> GSMGKPFFTRNPSELKGKFIHTKLRKSSRGFGFTVVGGDEPDEFLQIKSLVLDGPAALDGKMETGDVIVSVNDTCVLGHTHAQVVKIFQSIPIGASVDLELCRGYPLGSSAYGSVKAYTNFDAERDALNIETAIKTKGVDEVTIVNILTNRSNEQRQ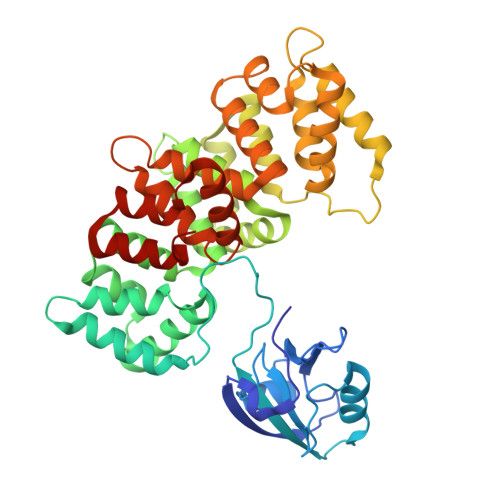DIAFAYQRRTKKELASALKSALSGHLETVILGLLKTPAQYDASELKASMKGLGTDEDSLIEIICSRTNQELQEINRVYKEMYKTDLEKDIISDTSGDFRKLMVALAKGRRAEDGSVIDYELIDQDARDLYDAGVKRKGTDVPKWISIMTERSVPHLQKVFDRYKSYSPYDMLESIRKEVKGDLENAFLNLVQCIQNKPLYFADRLYDSMKGKGTRDKVLIRIMVSRSEVDMLKIRSEFKRKYGKSLYYYIQQDTKGDYQKALLYLCGGDD[(4-ETHYLPHENYL)AMINO]CARBONYLPHOSPHONIC ACID | C9 H12 N O4 P | 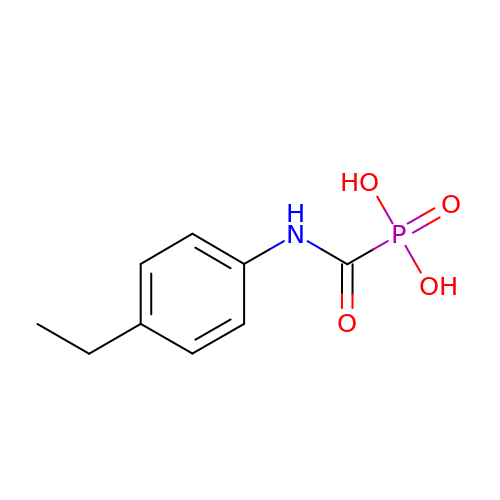KGNSYMGWPCEFDZ-UHFFFAOYSA-N>[2x]GARASVLSGGE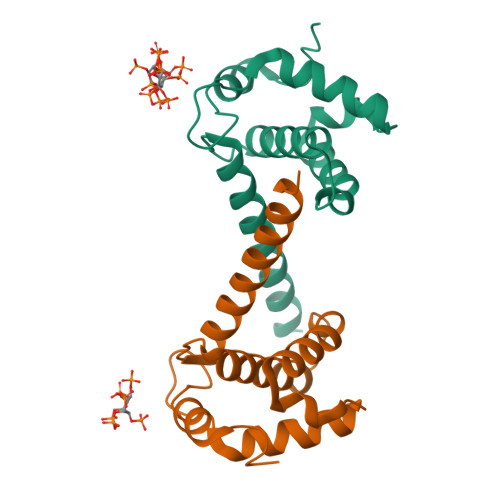LDKWEKIRLRPGGKKQYKLKHIVWASRELERFAVNPGLLETSEGCRQILGQLQPSLQTGSEELRSLYNTIAVLYCVHQRIDVKDTKEALDKIEEEQNKSKKKAQQAAADTG> PISPIETVPVKLKPGMDGPKVKQWPLTEEKIKALVEICTEMEKEGKISKIGPENPYNTPVFAIKKKDSTKWRKLVDFRELNKRTQDFWEVQLGIPHPAGLKKKKSVTVLDVGDAYFSVPLDEDFRKYTAFTIPSINNETPGIRYQYNVLPQGWKGSPAIFQSSMTKILEPFKKQNPDIVIYQYMDDLYVGSDLEIGQHRTK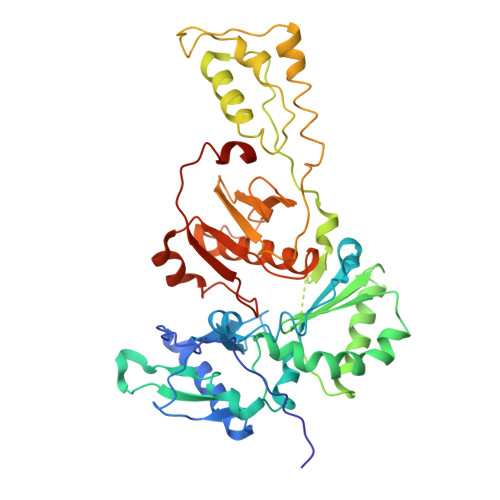IEELRQHLLRWGLTTPDKKHQKEPPFLWMGYELHPDKWTVQPIVLPEKDSWTVNDIQKLVGKLNWASQIYPGIKVRQLSKLLRGTKALTEVIPLTEEAELELAENREILKEPVHGVYYDPSKDLIAEIQKQGQGQWTYQIYQEPFKNLKTGKYARMRGAHTNDVKQLTEAVQKITTESIVIWGKTPKFKLPIQKETWETWWTEYWQATWIPEWEFVNTPPLVKLWYQLGGHHHHHH5-[(1~{S})-1-[4-azanyl-3-(5-oxidanylpyridin-3-yl)pyrazolo[3,4-d]pyrimidin-1-yl]ethyl]-4-cyclopentyl-2-(phenylmethyl)pyridazin-3-one | C28 H28 N8 O2 | 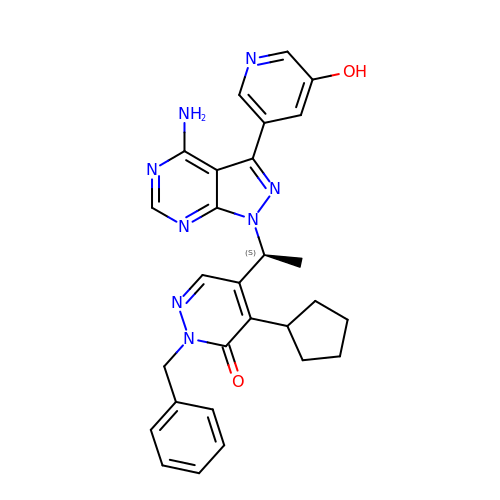DRNLTPZVKYHLED-KRWDZBQOSA-N>MVVNNKVDSLSYDVEAPPAQAPTTPAVVSAPPTPRGEAPAMTTTAAAELHKVSVPERRSTAKALRQRLAEVFFPDDPLHQFKNQSSARRLVLALQYFFPIFHWGSDYSLRLLRSDVVSGLTIASLAIPQGISYAKLANLPPIIGLYSSFVPPLIYSLLGSSRDLAVGPVSIASLVMGSMLRQAVSPDQEPILYLQLAFTSTFFAGVFQASLGFLRLGFIVDFLSKATLTGFMGGAAIIVSLQQLKGLLGIIHFTSQMGFVQVMHSVFKHHDEWAWQTILMGVAFLAVLLTTRHISARNPKLFWVSAAAPLTSVIISTIISFVSKAHGISVIGDLPKGLNPPSANMLTFSGSYVGLALNTGIMTGILSLTEGIAVGRTFASINNYQVDGNKEMMAIGVMNMAGSCASCYVTTGSFSRSAVNYSAGCKTAVSNIVMASAVLVTLLFLMPLFHYTPNVILSAIIITAVIGLIDVRGAARLWKVDKLDFLACMAAFLGVLLVSVQMGLAIAVGISLFKILLQVTRPNMVVKGVVPGTASYRSMAQYREAMRVPSFLVVGVESAIYFANSMYLGERIMRFLREEDERAAKCNQCPVRCIILDMSAVAAIDTSGLDALAELKKVLEKRNIELVLA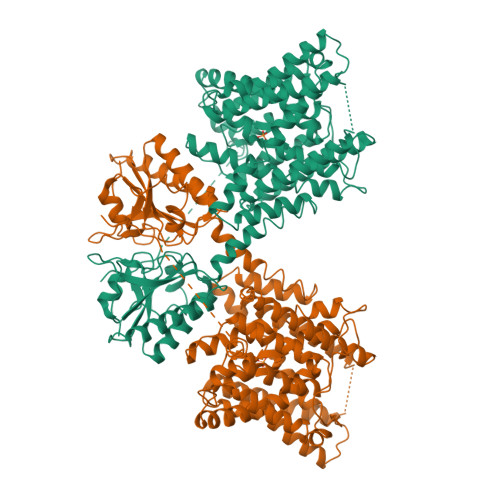NPVGSVTERLYNSVVGKTFGSDRVFFSVAEAVAAAPHKTQP[2x]(4Z)-4-({[(1E)-1-carboxy-3-(methylsulfanyl)propylidene]azaniumyl}methylidene)-2-methyl-5-[(phosphonooxy)methyl]-1,4-dihydropyridin-3-olate 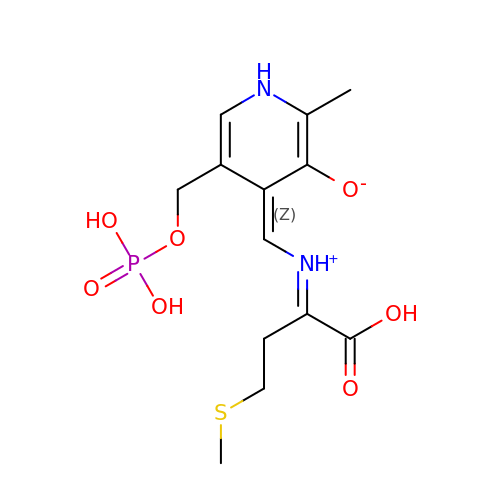| C13 H19 N2 O7 P S | UNHRYMFMFMQCNK-JNVWRRHBSA-N Abscisic acid (ABA) is a phytohormone essential to the regulation of numerous aspects of plant growth and development. ABCG25 in Arabidopsis thaliana has been identified to be an ABA exporter and play roles in regulating stomatal closure and seed germination. As a ‘half-transporter’ with only one NBD and one transmembrane domain (TMD) in a polypeptide chain, ABCG25 forms a homodimer as a functional unit, similar to other determined ‘half-transporter’ ABCG structures including the human cholesterol transporter ABCG1 (hABCG1) and multidrug transporter ABCG2 (hABCG2)39–47. In this study, we determined the high-resolution structures of ABCG25 in Arabidopsis thaliana in the apo, ABA-bound and ATP-bound states using cryogenic electron microscopy (cryo-EM) single particle analysis.

We also purified ABCG25WT protein with DDM extraction and ABA addition during the whole purification step, and finally determined an EM map with an overall resolution of 3.2 Å. The protein structure is almost identical to that determined with DDM plus CHS extraction, with an RMSD of 0.25 Å. A clear density was also observed in the identical site in protein sample prepared with DDM plus CHS, which can be docked by one ABA molecule with a better fitting density, further supporting the ABA binding site. ABA lies almost at the middle of the TMDs, with the carboxylate tail pointing to the bottom of the cavity and the ring head group pointing to the cytoplasmic side. The interface between ABA and ABCG25 is mainly formed by TM2 and TM5a. The surrounding residues are hydrophobic or polar in nature, including Q413 on TM1; F442, I445, V449 and F453 on TM2 of one subunit; and T552, L556 and V559 on TM5 of the other subunit. The phenolic hydroxyl groups of Y565 form a hydrogen bond with the carboxylate group of ABA, and Q413 interacts with the ketone group of the cyclohexene ring. In addition, as in the apo-state structure, Y565, Y564 and H434 seal the TMD to the extracellular space and form a gate for ABA release.

>[2x]MSAFDGVENQMNGPDSSPRLSQDPREPRSLLSSSCFPITLKFVDVCYRVKIHGMSNDSCNIKKLLGLKQKPSDETRSTEERTILSGVTGMISPGEFMAVLGPSGSGKSTLLNAVAGRLHGSNLTGKILINDGKITKQTLKRTGFVAQDDLLYPHLTVRETLVFVALLRLPRSLTRDVKLRAAESVISELGLTKCENTVVGNTFIRGISGGERKRVSIAHELLINPSLLVLDEPTSGLDATAALRLVQTLAGLAHGKGKTVVTSIHQPSSRVFQMFDTVLLLSEGKCLFVGKGRDAMAYFESVGFSPAFPMNPADFLLDLANGVCQTDGVTEREKPNVRQTLVTAYDTLLAPQVKTCIEVSHFPQDNARFVKTRVNGGGITTCIATWFSQLCILLHRLLKERRHESFDLLRIFQVVAASILCGLMWWHSDYRDVHDRLGLLFFISIFWGVLPSFNAVFTFPQERAIFTRERASGMYTLSSYFMAHVLGSLSMELVLPASFLTFTYWMVYLRPGIVPFLLTLSVLLLYVLASQGLGLALGAAIMDAKKASTIVTVTMLAFVLTGGYYVNKVPSGMVWMKYVSTTFYCYRLLVAIQYGSGEEILRMLGCDSKGKQGASAATSAGCRFVEEEVIGDVGMWTSVGVLFLMFFGYRVLAYLALRRIKH>PQTEEVSIKEIAITHHVKEGHEKADPSQFELLKVLGQGSFGKVFLVKKISGSDARQLYAMKVLKKATLKVRDRVRTKMERDILVEVNHPFIVKLHYAFQTEGKLYLILDFLRGGDLFTRLSKEVMFTEEDVKFYLAELALALDHLHSLGIIYRDLKPENILLDEEGHIKLTDFGLSKESIDHEKKAYSFCGTVEYMAPEVVNRRGHTQSADWWSFGVLMFEMLTGTLPFQGKDRKET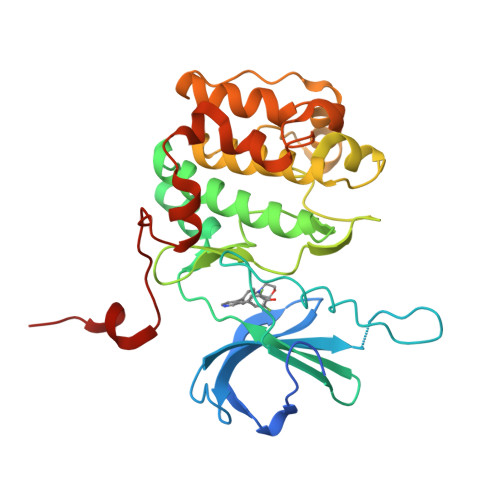MTMILKAKLGMPQFLSPEAQSLLRMLFKRNPANRLGAGPDGVEEIKRHSFFSTIDWNKLYRREIHPPFKPATGRPEDTFYFDP[10x]> GSHMPDPAAHLPFFYGSISRAEAEEHLKLAGMADGLFLLRQCLRSLGGYVLSLVHDVRFHHFPIERQLNGTYAIAGGKAHCGPAELCEFYSRDPDGLPCNLRKPCNRPSGLEPQPGVFDCLRDAMVRDYVRQTWKLEGEALEQAIISQAPQVEKLIATTAHERMPW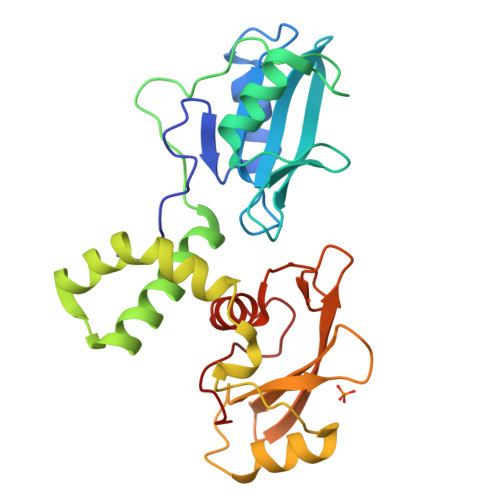YHSSLTREEAERKLYSGAQTDGKFLLRPRKEQGTYALSLIYGKTVYHYLISQDKAGKYCIPEGTKFDTLWQLVEYLKLKADGLIYCLKEACPN> MKNTIHINSNDSVTLRLMTEHDLAMLYEWLNRSHIVEWWGGEEARPTLADVQEQYLPSVLAQESV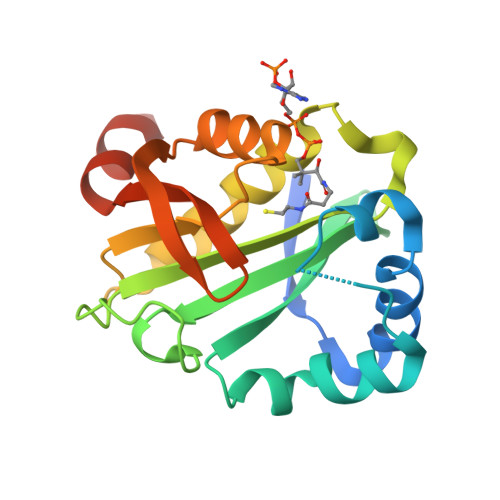TPYIAMLNGEPIGYAQSYVALGSGDGWWEEETDPGVRGIDQLLANASQLGKGLGTKLVRALVELLFNDPEVTKIQTDPSPSNLRAIRCYEKAGFERQGTVTTPDGPAVYMVQTRQAFERTRSDEGRAQFEA>[2x]MATEKHFKYVVLGGGVAGGYAAREFAKQGVQPGELAIISREAVAPYERPALSKAYLFPQNPARLPGFHVCVGSGGERLLPEWYSEKGIELILN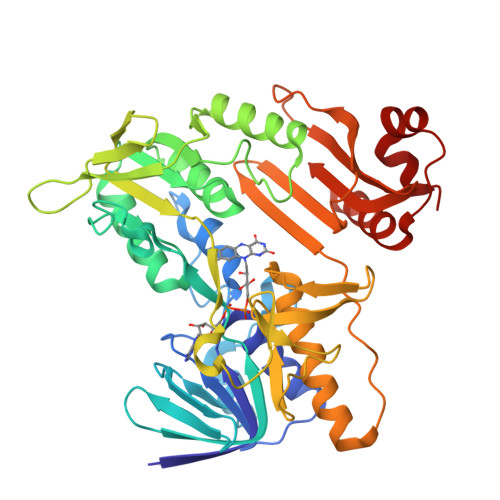TEIVKADLASKTLTSAAGATFTYEILLIATGSSVIKLSDFGTQGADSNNILYLREVDDADKLYAAIQAKKGGKAVVVGGGYIGLELSAVLKMNNLDVTMVFPEPWCMPRLFTAEIAAFYESYYTNKGVKIVKGTVAVGFDADANGDVTAVKLKDGSVLEADIVVVGVGGRPLTTLFKGQVAEEKGGIKTDASFETSVPGVYAVGDVATFPMKIYNDVRRVEHVDHSRKSAEQAVKAIKGKESGEAVPEYDYLPYFYSRSFDLSWQFYGDNVGEAVLFGDSDPASAKPKFGSYWIKDGKVVGAFLEGGSGDENGLIAKVARAQPPVSSIEELKQDGLLFASKI> MELIGDYSKAFLLQTVDGKHQDLKYISPETMVALLTGKFSNIVDKFVIVDCRYPYEYEGGHIKTAVNLPLERDAESFLLKSPIAPCSLDKRVI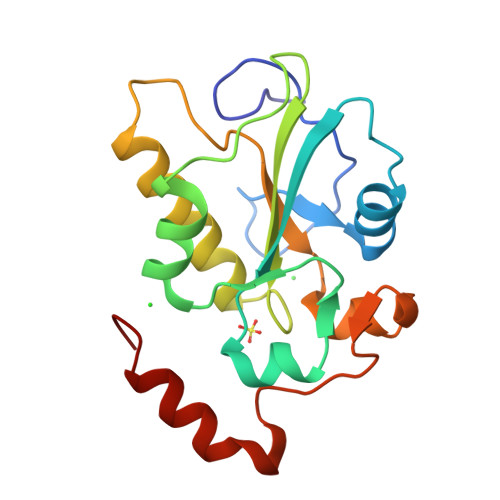LIFHCEFSSERGPRMCRFIRERDLAVNDYPSLYYPEMYILKGGYKEFFPQHPNFCEPQDYRPMNHEAFKDELKTFRLKTRSW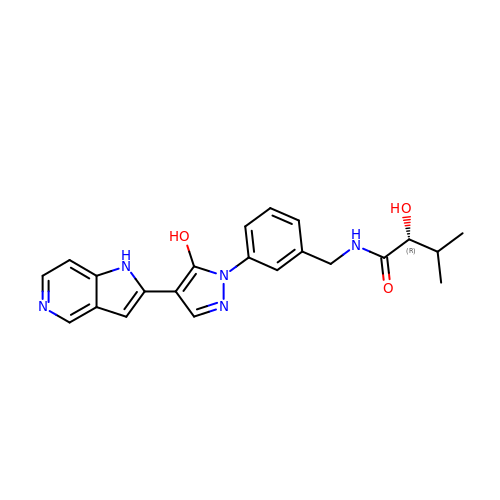(2R)-2-hydroxy-N-[[3-[5-hydroxy-4-(1H-pyrrolo[3,2-c]pyridin-2-yl)pyrazol-1-yl]phenyl]methyl]-3-methylbutanamide | C22 H23 N5 O3 | HYHVHHKEOHYVCZ-HXUWFJFHSA-N>MSIKIRDFGLGSDLISLTNKAGVTISFTNLGARIVDWQKDGKHLILGFDSAKEYLEKDAYPGATVGPTAGRIKDGLVKISGKDYILNQNEGPQTLHG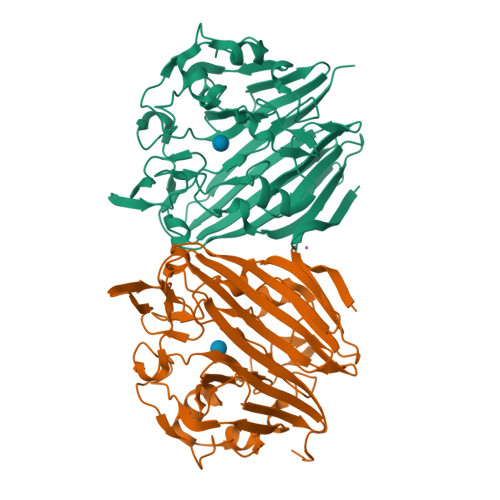GEESIHTKLWTYEVTDLGAEVQVKFSLVSNDGTNGYPGKIEMSVTHSFDDDNKWKIHYEAISDKDTVFNPTGHVYFNLNGDASESVENHGLRLAASRFVPLKDQTEIVRGDIVDIKNTDLDFRQEKQLSNAFNSNMEQVQLVKGIDHPFLLDQLGLDKEQARLTLDDTSISVFTDQPSIVIFTANFGDLGTLYHEKKQVHHGGITFECQVSPGSEQIPELGDISLKAGEKYQATTIYSLHTKLEHHHHHH[2x]> MAMLESAVDSAAFADDDVQASPPHAVTGYRSFQLGAFELSRDEYFARITWPAKGETRSHLIPADIFLRAMMRDVAWGFFYGWVNFDHVIGTRNYYGKVDLYAGTFNGTLKAAGVNYTENFETPLIMATFKAILRDWTNATFDPFAAPEETGSAFGRKNGENLECIERFRIATKR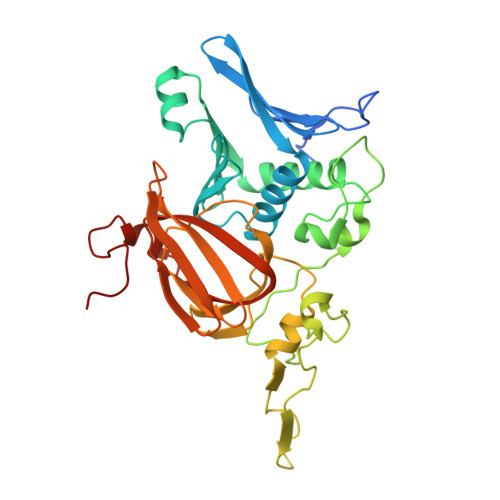MPGLQDDSPLRNDLPVNRQFADVSQDEPEVHAAEGFEGELHAFSLFKYLSRSDVTWNPSVTSVCKASLFCPTTEEFILPVFHGNDRVEWFIQMSDEIVWDVGDKDDGNPRARITMRAGDVCAMPADIRHQGYSTKRSMLMVWENATPNLPHLYESGELKPYPIEF> MGRALSAWVGYSVLGAVLDPTGKIVERFTPEVAPISEERVIDVAPPSYASRVGVREPLITGVRAIDGLLTCGVGQRMGIFASAGCGKTMLMHMLIEQT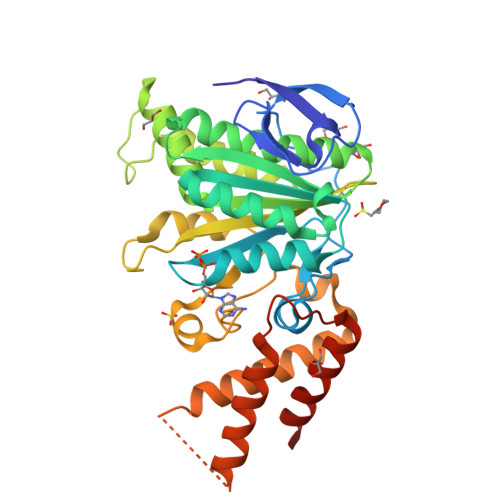EADVFVIGLIGERGREVTEFVDMLRASHKKEKCVLVFATSDFPSVDRCNAAQLATTVAEYFRDQGKRVVLFIDSMTRYARALRDVALASGERPARRGYPASVFDNLPRLLERPGATSEGSITAFYTVLLESEEEADPMADEIRSILDGHLYLSRKLAGQGHYPAIDVLKSVSRVFGQVTTPTHAEQASAVRKLMTRLEELQLFIDLGEYRPGENIDNDRAMQMRDSLKAWLCQPVAQYSSFDDTLSGMNAFADQNSAWSHPQFEK>[2x]MRRSGNYNPSRWDVNFIQSLLSDYKEDKHVIRASELVTLVKMELEKETDQIRQLELIDDLQRMGLSDHFQNEFKEILSSIYLDHHYYKNPFPKEERDLYSTSLAFRLLREHGFQVAQEVFDSFKNEEGEFKESLSDDTRGLLQLYEASFLLTEGETTLESAREFATKFLEEKVNEGGVDGDLLTRIAYSLDIPLHWRIKRPNAPVWIEWYRKRPDMNPVVLELAILDLNIVQAQFQEELKESFRWWRNTGFVEKLPFARDRLVECYFWNTGIIEPRQHASARIMMGKVNALITVIDDIYDVYGTLEELEQFTDLIRRWDINSIDQLPDYMQLCFLALNNFVDDTSYDVMKEKGVNVIPYLRQSWVDLADKYMVEARWFYGGHKPSLEEYLENSWQSISGPCMLT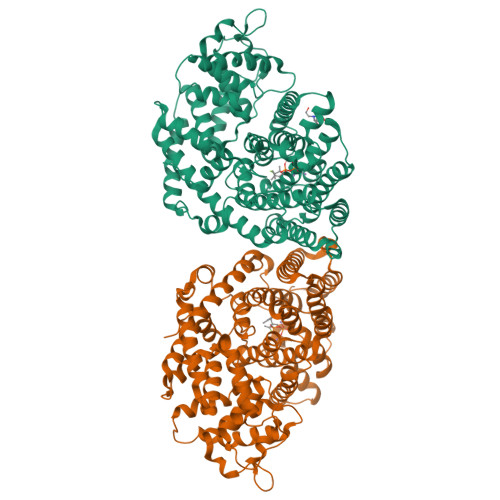HIFFRVTDSFTKETVDSLYKYHDLVRWSSFVLRLADDLGTSVEEVSRGDVPKSLQCYMSDYNASEAEARKHVKWLIAEVWKKMNAERVSKDSPFGKDFIGCAVDLGRMAQLMYHNGDGHGTQHPIIHQQMTRTLFEPFA> GPLGSMPGFSQATELGAWKELQEHHNSLGRNIVLKEYFEKDPQRFEKFSRTFANPVDNTEILFDFSKNFLTEETLALLVKLAREAGVEELRDAMFKGDPINFTEDRAVYHVALRNVTNEPMQVNGKSVVEDVNSVLEHMKEFTEQVRSGEWKGYTGKKITTIINIGIGGSDLGPVMVTEALKPYGAEDMTLHFVSNIDGSHIAEALKHSDPETTLFLIASKTFTTAETTTNA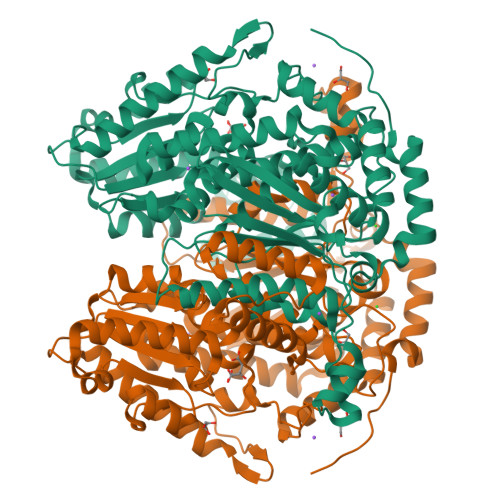NSAKKWFLESAKDEAHIAKHFVALSTNEEEVTKFGIDKKNMFGFASWVGGRYSVWSAIGLSVALYIGFDNFHQFLAGAHAMDKHFRETPLEQNIPVLGGLLSVWYSDFFGAQTHLVAPFDQYLHRFPAYLQQLSMESNGKAITRTGEYVKYTTGPILFGEPATNAQHSFFQLLHQGTKLIPSDFIMAAESHNPVEGGKHQRMLASNFLAQSEALMVGKTPEQVKTEGAPDNLVPHKTFLGNRPTTSILAQKITPSTLGALIAYYEHLTFTEGAVWNINSFDQWGVELGKVLAKKIQKELETPGAGGDHDASTSGLLLAFKKKANLA4-benzoylbenzoic acid | C14 H10 O3 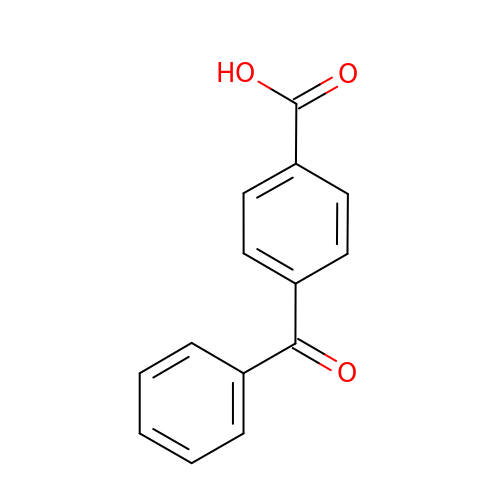| IFQUPKAISSPFTE-UHFFFAOYSA-N>[2x]MAVLKIISWNVNGLRAVHRKGFLKWFMEEKPDILCLQEIKAAPEQLPRKLRHVEGYRSFFTPAERKGYSGVAMYTKVPPSSLREGFGVERFDTEGRIQIADFDDFLLYNIYFPNGKMSEERLKYKLEFYDAFLEDVNRERDSGRNVIICGDFNTAHREIDLARPKENSNVSGFLPVERAWIDKFIENGYVDTFRMFNSDPGQYTWWSYRTRARERNVGWRLDYFFVNEE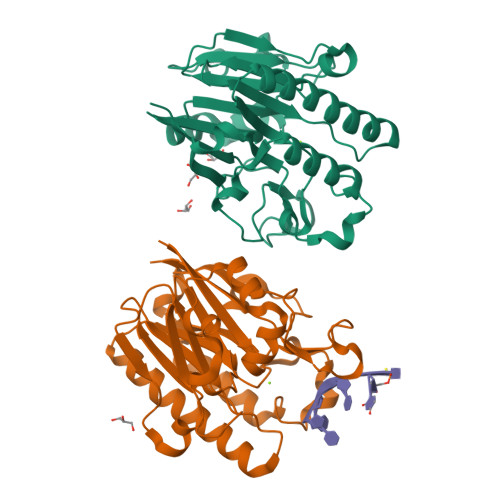FKGKVKRSWILSDVMGSDHCPIGLEIELLEHHHHHH> ADPHHHHHHHHPVTPCEAPLQWEGRIVLYDHNTGKNTRATVTYDAILQRIRILEE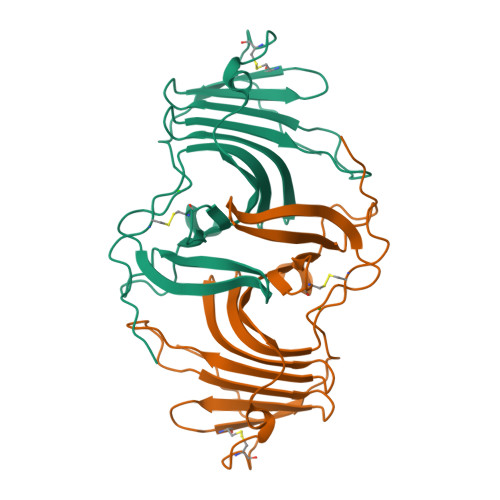KKSFVPCKRFFEYIFLYQEAVMFQIEQVTKICSKNTLTEPWDPYDIPENSTYEDQYYIGGPGDQIPVQEWSDRKPARKYETWVGVYTVKDCYPVQETYTKNDSMTTSTRFFDIKLGISDPSVFNPPSTCEAAQPLLMSGDC>MGAQETIVIGLAADSGCGKSTFMRRLTSVFGGAAKPPKGGNPDSNTLISDTTTVICLDDYHSLDRYGRKEQKVTALDPRANDFDLMYEQVKALKNGIAVEKPIYNHVTGLLDPPELIQPPKILVIEGLHPMFDERVRDLLDFSIYLDISNEVKFAWKIQRDMAERGHSLESIKASIEARKPDFDAFIDPQKQYADAVIEVLPTTLIPDDNEGKVLRVRLIMKEGVKYFSPVYLFDEGSTISWIPCGRKLTCSYPGIKFNYEPDSYFDHEVSVLEMDGQFDRLDELIYVESHLSNLSTKFYGEVTQQMLKHADFPGSNNGTGLFQTI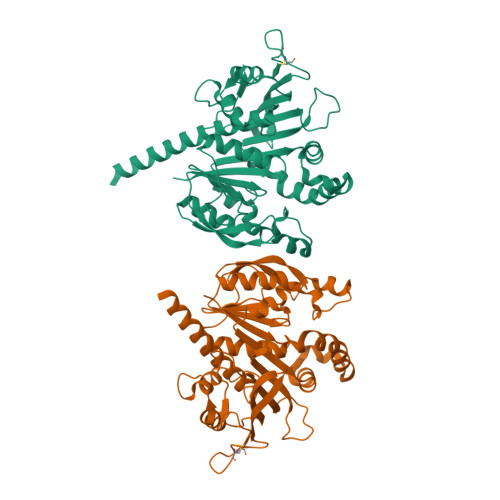VGLKIRDLYEQLIANKATARAEAKALEHHHHHH[4x]>MNAQAEEFKKYLETNGIKPKQFHKKELIFNQWDPQEYCIFLYDGITKLTSISENGTIMNLQYYKGAFVIMSGFIDTETSVGYYNLEVISEQATAYVIKINELKELLSKNLTHFFYVFQTLQKQVSYSLAKFNDFSING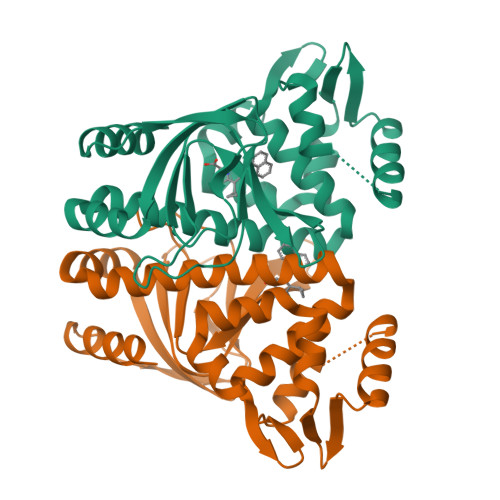KLGSICGQLLILTYVYGKETPDGIKITLDNLTMQELGYSSGIAHSSAVSRIISKLKQEKVIVYKNSCFYVQNLDYLKRYAPKLDEWFYLACPATWGKLN[2x]>TVEAKNETFAPQHPDQYLSWKATSEQSERVDALAEDPRLVILWAGYPFSRDYNKPRGHAFAVTDVRETLRTGAPKNAEDGPLPMACWSCKSPDVARLIQKDGEDGYFHGKWARGGPEIVNNLGCADCHNTASPEFAKGKPELTLSRPYAARAMEAIGKPFEKAGRFDQQSMVCGQCHVEYYFDGKNKAVKFPWDDGMKVENMEQYYDKIAFSDWTNSLSKTPMLKAEHPEYETWTAGIHGKNNVTCIDCHMPKVQNAEGKLY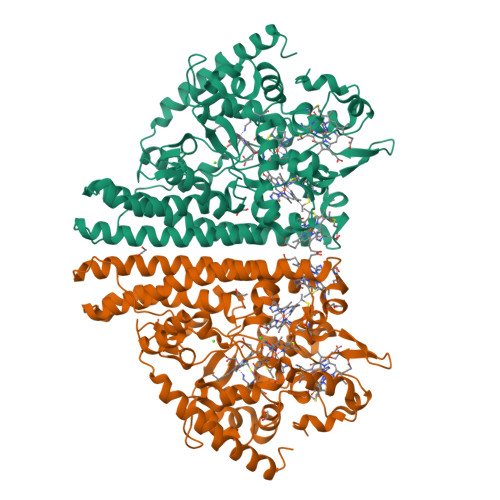TDHKIGNPFDNFAQTCANCHTQDKAALQKVVAERKQSINDLKIKVEDQLVHAHFEAKAALDAGATEAEMKPIQDDIRHAQWRWDLAIASHGIHMHAPEEGLRMLGTAMDKAADARTKLARLLATKGITHEIQIPDISTKEKAQQAIGLNMEQIKAEKQDFIKTVIPQWEEQARKNGLLS[4x]>[3x]SREFDFFTYETPKVIVVKSWTIGIINRVVQLLIISYFVGWVFLHEKAYQVRDTAIESSVVTKVKGSGLYANRVMDVSDYVTPPQGTSVFVIITKMIVTENQMQGFCPESEEKYRCVSDSQCGPERLPGGGILTGRCVNYSSVLRTCEIQGWCPTEVDTVETPIMMEAENFTIFIKNSIRFPLFNFEKGNLLPNLTARDMKTCRFHPDKDPFCPILRVGDVVKFAGQDFAKLARTGGVLGIKIGWVCDLDKAWDQCIPKYSFTRLDSVSEKSSVSPGYNFRFAKYYKMENGSEYRTLLKAFGIRFDVLVYGNAGKFNIIPTIISSVAAFTSVGVGTVLCDIILLNFLKGADQYKAKKFEEVNE

P2X3 receptors are a family of trimeric cation channels that are activated by extracellular ATP. They play particularly important roles in sensory neurons where their activation is critical for gustatory and nociceptive responses (Barclay et al., 2002; Chen et al., 1995; Cook et al., 1997; Finger et al., 2005; Huang et al., 2011; North, 2003; North, 2004; Vandenbeuch et al., 2015), visceral reflexes and sensory hypersensitization. P2X3 homomeric receptors activate and desensitize on the millisecond timescale upon binding ATP but unbind ATP and recover from desensitization on the timescale of minutes. Although free-ATP is an agonist in laboratory conditions, P2X3 receptors are activated primarily by Ca2+-ATP and Mg2+-ATP under physiological conditions because ATP released from cells at micromolar concentrations would largely be in complex with Ca2+ and Mg2+, both of which are present in millimolar concentrations in extracellular physiological solutions.

We began by crystalizing the hP2X3 MFCslow construct in solutions containing ATP with either Mg2+ or Ca2+. We solved X-ray structures of the receptor with Mg2+-ATP or Ca2+-ATP bound at resolutions of 3.8 Å and 3.3 Å, respectively. The pores appear to be in an open-like conformation in both structures, similar to that observed in the structure of hP2X3 bound to free-ATP. Importantly, we observed strong residual electron densities around the ATP binding site in these structures. Considering that the crystallization conditions included either 50 mM Mg-acetate or 50 mM Ca-acetate with no other divalent cations, and that the electron densities are surrounded by acidic residues, we interpreted the densities as Mg2+ and Ca2+ ions, respectively. In both structures, the divalent ions are detected at the edge of the ATP binding pocket, simultaneously interacting with D158 on the receptor and with the γ-phosphate of ATP; E156 is also positioned nearby and appears to be involved in coordinating the ion. Conversely, in our ATP-bound structure, with Mg2+ directly coordinated by the ATP γ-phosphate and D158, the ion is ~9 Å away from the side chain of E109. The key residue involved in both binding modes is D158, whose side chain points towards E109 for the upper mode or towards the γ-phosphate of ATP for the lower mode. That the Mg2+-ATP complex observed in our structures adopts a rare configuration suggests that interactions between the receptor and divalent ions have a dominant effect in determining the structure and stability of the complex. In the presence of ATP and Mg2+, the simulation data (obtained with a conventional algorithm) is highly consistent with our crystal structures, showing stable close-range interactions between Mg2+ and both the ATP γ-phosphate and D158.>[2x]MFKDGSLIPYLTAGDPDKQSTLNFLLALDEYAGAIELGIPFSDPIADGKTIQESHYRALKNGFKLREAFWIVKEFRRHSSTPIVLMTYYNPIYRAGVRNFL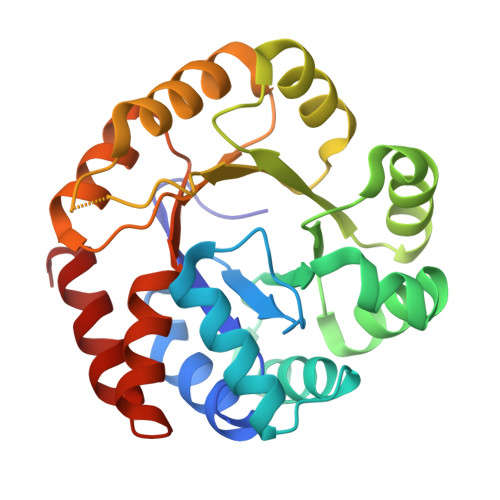AEAKASGVDGILVVDLPVFHAKEFTEIARAAGIKTVFLAAPNTPDERLKVIDDMTTGFVYLVSLYGTTGAREEIPKTAYDLLRRAKRICRNKVAVGFGVSKREHVVSLLKEGANGVVVGSALVKIIGEKGREATEFLKKKVEELLGI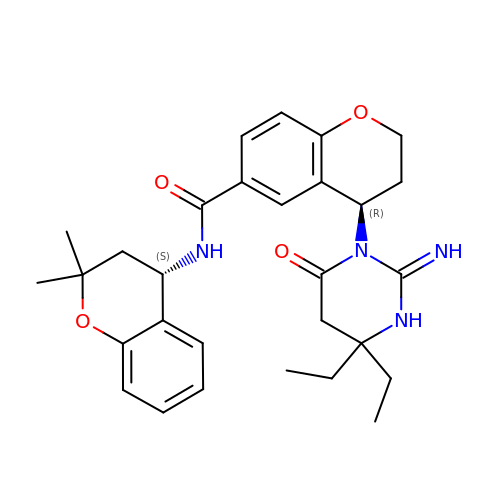(4R)-4-[(2E)-4,4-diethyl-2-imino-6-oxo-1,3-diazinan-1-yl]-N-[(4S)-2,2-dimethyl-3,4-dihydro-2H-1-benzopyran-4-yl]-3,4-dihydro-2H-1-benzopyran-6-carboxamide | C29 H36 N4 O4 | ZSZSSSHEMYULPX-FCHUYYIVSA-N Lipin/Pah phosphatidic acid phosphatases (PAPs) are Mg2+-dependent enzymes that catalyze the dephosphorylation of phosphatidic acid (PA) to produce diacylglycerol. pmcLipin/Pah phosphatidic acid phosphatases (PAPs) are magnesium-dependent enzymes that are evolutionarily conserved from yeast to humans. They catalyze the penultimate step of triacylglycerol synthesis, through the conversion of phosphatidic acid (PA) to diacylglycerol (DAG). Structurally, all lipin/Pah PAPs contain highly conserved N-Lip and C-Lip regions that combine to form two domains: an immunoglobulin-like (Ig-like) domain and a HAD-like catalytic domain. The remainder of the C-Lip adopts a Rossmann-fold, forming the haloacid dehalogenase-like (HAD-like) domain and harbors a conserved catalytic motif DxDxT, where the first Asp coordinates a Mg2+ ion that increases its nucleophilicity, and the second Asp participates in acid/base catalysis.

Structure 5 was determined using a construct that retained the N-terminal helix but contained a D155N point mutant. This point mutant was originally designed for enzymatic assays to probe the role of D155 in catalysis and substrate recognition, as it was found to play a role in magnesium coordination in structures 3 and 4. Other HAD phosphatases have similar magnesium coordination, however we sought to increase our confidence in our modeling by determining the structure of a D155N point mutant. This structure (Structure 5) was determined in the presence of calcium. Notably, there was no observable electron density for the entire D155N residue, and the sixth coordination site of calcium was now occupied by a serine residue from the N-terminal helix from an adjacent molecule in the asymmetric unit. Crystal packing involved interactions of the N-terminal helix with another molecule, with the N-terminal helix partially ordered in this structure. Overall, we concluded that Tt Pah2 coordinates magnesium using Asp155, in addition to other canonical residues in the HAD superfamily.

>[2x]MINGIKNLFSYLFDSKDYSTFSGVVDIIVVRQPDDSLKSMPFHIRFGTLKVLDNQNINIQITVNDKKIEDVFMLMLPEGACYFPELNAKNEIQKKLRPSSAILKKFNLKNGYNKIQFIAESDLQGKQLIEGKIYLYNYDTKLVISDVDGTVTKSNVKGHISTIIGKEWTHDDIAELYTNIQKNGYKMVYLSSRPLYFYNYTQGYLKGIIQNGFTMPDGPILLSPDQIISSLNREVVYKKADEFKGALLKDLRRVFPEEVNPIFAGFGNRDTDATACLYAGVIIDNIFIINEQSQVEILGKQEKSSYKKINEKIQELFPRLP2-azanylidene-N-(3-ethylphenyl)-8-oxidanyl-chromene-3-carboxamide | C18 H16 N2 O3 | 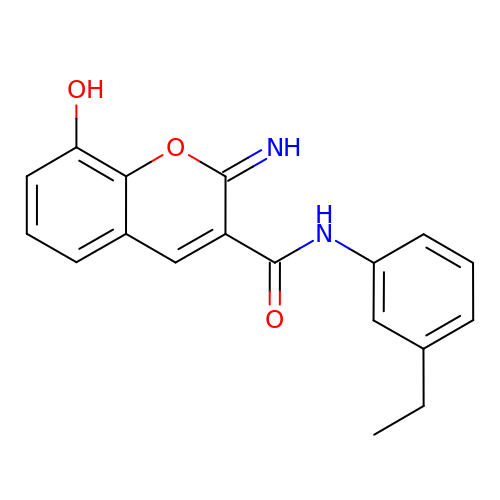KJSIIAIZHJYKDK-ZPHPHTNESA-N> MAHHHHHHMTSVGLIWAQSTSGVIGRDGGIPWRLPEDLAHFKRLTMGHTVVMGRRTWDSLPAAHRPLPGRRNVVVTRQTGLVAHGAQVVGSLEQALSPAEPDAATWVIGGAQIYALALPLANRCEVTEVDVDLPPEDEDALAPVLDQ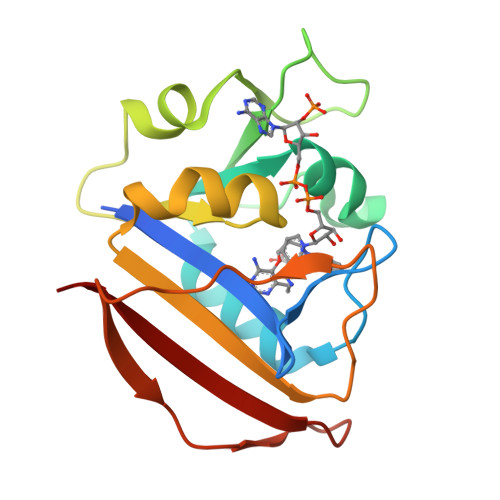TWAGTSGEWLVSRSGLRYRMHSYRRL(8S)-2-{[(4-tert-butylphenyl)methyl]amino}-5-[(piperidin-1-yl)methyl][1,2,4]triazolo[1,5-a]pyrimidin-7(6H)-one 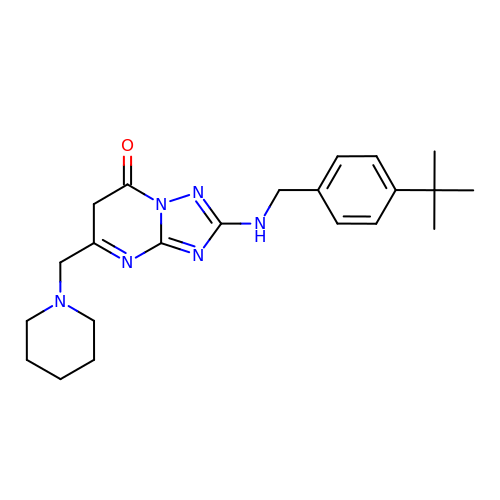| C22 H30 N6 O | OMZHFYCGCCKSTE-UHFFFAOYSA-N> GPLGSVRDEIRSMVSDSVDEIVDGVSKTTAEVINGRKSIAQYATSLIESNPEPDNVRTIISQPLIKNTFLLVGFGLEKDGSNINNDPSWNPGPTWDPRVRPWYKDAKNAGKLVITAPYADSASGEILVSVATPVKDSATGQFLGSIFYDVSLAELAELVNEVKLFDAGYVFIVSEDGTTIAHPKKEFNGKPMSEFLGESKINVDTHQVIINGKPYAVSFSDV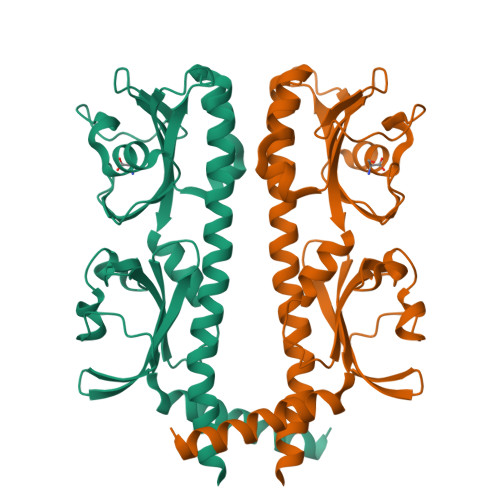EGEDWYVGVVIDEEIAYAALDELRRSTLIHHHHHH Drosophila ROS1 (dROS1), also known as Sevenless, is a critical RTK required for R7 photoreceptor development. Like all other RTKs, the architecture of dROS1 is composed of an extracellular region (ECR), a single-pass transmembrane domain (TM), and an intracellular kinase domain (KD). Here we show, the extracellular region of dROS1 adopts a folded-over conformation stabilized by an N-terminal domain comprised of two disulfide stapled helical hairpins.

We expressed and purified the dROS1 ECR (construct 1–6) and obtained a 3.94 Å structure using single-particle CryoEM. Surprisingly, model building only resolves the N-terminal region (equivalent to construct 1-4) starting from the N-terminus to the fourth FNIII domain. The C-terminal domains starting from the fifth FNIII domain to the sixth, including the intervening YWTD-C, were not observed in the map. The lack of density for the C-terminal domains is consistent with this region demonstrating greater flexible with respect to the N-terminal domains. Interestingly, the model reveals that rather than having a linear arrangement of domains, the N-terminal region adopts a folded-over conformation stabilized by an interaction of an N-terminal cysteine-rich region with the second propeller (YWTD-B) and fourth FNIII domain. The domain is comprised of two disulfide stapled helical hairpins that associate with one another through hydrophobic interactions. The two helical hairpins generate two loops (capping loops 1 and 2) which stabilize the N-terminal ECR compacted fold. In the loop generated by the first helical hairpin, capping loop 1, F235 sits between R1234 and L1236 of the fourth FNIII domain. F231 sits between R1032 and L1034 of the second propeller. Our structure, of dROS1’s N-terminal ECR—being compact rather than linear, suggests that the bulky ECR could physically keep the kinase domain at distance and prevent oligomerization and signaling in the absence of ligand binding.

> HHHHHHHHGSSTSNIEGRSRVTRDCVQRCIVEEDLFLDEFGIQCEKADNGEKCYKTRCTKGCAQWYRALKELESCQEACLSLQFYPYDMPCIGACEMAQRDYWHLQRLAISHLVERTQPQLERAPRADGQSTPLTIRWAMHFPEHYLASRPFNIQYQFVDHHGEELDLEQEDQDASGETGSSAWFNLADYDCDEYYVCEILEALIPYTQYRFRFELPFGENRDEVLYSPATPAYQTPPEGAPISAPVIEHLMGLDDSHLAVHWHPGRFTNGPIEGYRLRLSSSEGNATSEQLVPAGRGSYIFSQLQAGTNYTLALSMINKQGEGPVAKGFVQTHSARNEKPAKDLTESVLLVGRRAVMWQSLEPAGENSMIYQSQEELADIAWSKREQQLWLLNVHGELRSLKFESGQMVSPAQQLKLDLGNISSGRWVPRRLSFDWLHHRLYFAMESPERNQSSFQIISTDLLGESAQKVGESFDLPVEQLEVDALNGWIFWRNEESLWRQDLHGRMIHRLLRIRQPGWFLVQPQHFIIHLMLPQEGKFLEISYDGGFKHPLPLPPPSNGAGNGPASSHWQSFALLGRSLLLPDSGQLILVEQQGQAASPSASWPLKNLPDCWAVILLVPESQPLTSAGGKPHSLKALLGAQAAKISWKEPERNPYQSADAARSWSYELEVLDVASQSAFSIRNIRGPIFGLQRLQPDNLYQLRVRAINVDGEPGEWTEPLAARTWPLGPHRLRWASRQGSVIHTNELGEGLEVQQEQLERLPGPMTMVNESVGYYVTGDGLLHCINLVHSQWGCPISEPLQHVGSVTYDWRGGRVYWTDLARNCVVRMDPWSGSRELLPVFEANFLALDPRQGHLYYATSSQLSRHGSTPDEAVTYYRVNGLEGSIASFVLDTQQDQLFWLVKGSGALRLYRAPLTAGGDSLQMIQQIKGVFQAVPDSLQLLRPLGALLWLERSGRRARLVRLAAPLDVMELPTPDQASPASALQLLDPQPLPPRDEGVIPMTVLPDSVRLDDGHWDDFHVRWQPSTSGGNHSVSYRLLLEFGQRLQTLDLSTPFARLTQLPQAQLQLKISITPRTAWRSGDTTRVQLTTPPVAPSQPRRLRVFVERLATALQEANVSAVLRWDAPEQGQEAPMQALEYHISCWVGSELHEELRLNQSALEARVEHLQPDQTYHFQVEARVAATGAAAGAASHALHVAPEVQAVPRVLYANAEFIGELDLDTRNRRRLVHTASPVEHLVGIEGEQRLLWVNEHVELLTHVPGSAPAKLARMRAEVLALAVDWIQRIVYWAELDATAPQAAIIYRLDLCNFEGKILQGERVWSTPRGRLLKDLVALPQAQSLIWLEYEQGSPRNGSLRGRNLTDGSELEWATVQPLIRLHAGSLEPGSETLNLVDNQGKLCVYDVARQLCTASALRAQLNLLGEDSIAGQLAQDSGYLYAVKNWSIRAYGRRRQQLEYTVELEPEEVRLLQAHNYQAYPPKNCLLLPSSGGSLLKATDCEEQRCLLNLPMITASEDCPLPIPGVRYQLNLTLARGPGSEEHDHGVEPLGQWLLGAGESLNLTDLLPFTRYRVSGILSSFYQKKLALPTLVLAPLELLTASATDYKDDDDK> MQNGVFTRENADFLVKSGADSPSSQSLLLRTSPSPLSLP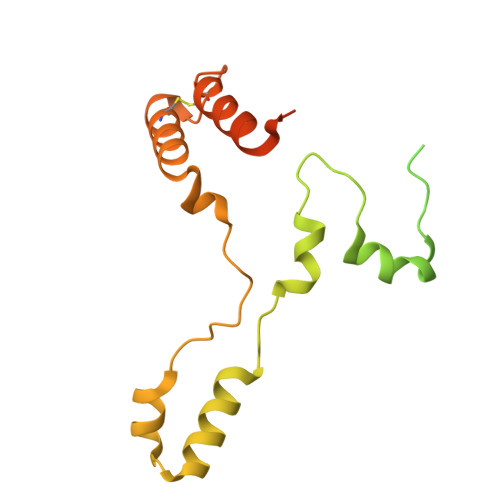RRRFIFLRSASVDLSERSSLACLAPFFCLASGVCLRSAFSLPFFARRGRPCLFFIFIFFFRVSFTANFRGKRVKMAASTIPISQWPSLLYAPPSSPANPAVEALPEMQFDDLHYPRQMLLCRGAGYSLEQCNRMAQPDARVTPENPAEKLLKEEAVAAIACLSQREGGKDEQCRYYIERMYKLANKEKQPEPGTLSKASTLACKLLGIHRPEA>[2x]MPSLPTLQPLDLYRRTLACLVLAVSCLGGGGLWADDARTSIEQRS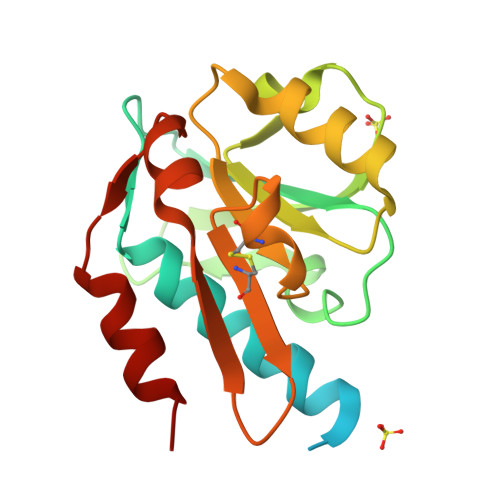NAVSQVLLGIFSYVRWPKEPAVLQLCVVGPTEYADGLLRGMVQANGRRVHAERRAVDNPDLGTLCNVIYLGVVDERERQQVFRSLAGHPVLSISERGTECSVGSMFCLNVGGPRITFEANLDSIARSGVRVHPSVLKLARRQATP> MRSMRALSLSLSIFAGAAVATTESTGKASIHDLALQKWTVTNEYGNITVPGKFPSQAHLDLHAAGVIGESNNGLNDFDLRWIAAQNWTYTSKPISGLSKHSDIATWLVFDGLDTYATVKFCDHIVGTPDNQFRQWFYDVSSALASCKSDPVLSINFGSVPRIINAINASDEVQHWPASVVYPFEYPNRQWVRKEQNDFGWDWGPAFSPVGPWQPGRIVQLSKGGELYSLNTDIDIFRKGQFNNFAPDQTAPWVVNASLDFLGTLPKHASMSVIITDASDSRSVLYSGKLEGVTQSDMTVTGSVTIDAHKPKLWWPRDMGNQQLYNITVSVSSAGSKTPILVSQRRVGFRTILFSSGNITDAQIASGITPGNNWHFEINGHEFYAKGANLIPPDAFWPRVTSDRMNRLFDSVESQNFNMLRVWSSGTYLPDWIYDIADERGVLLWSEFQFSDTLYPDSDDFKANVVGEITYNVRRLNHHASLACWMGGNEFENLMLPIAQGADPATYPYVLGQYENLFITTLFNVLAANSHSISYSPCSANNGWLEIDLDLPVPIVERYYNTTSGHIYGDTDFYNYDTSVSFDTSAYPVGRFANEFGFISMPSIQTWQQAVDPEELSFNSTTVILRNHHYPAGGLTRNIHNSTLGQVEMTLAVERYYPTPDKTDPVANFSSWCHATQLFQADMYKSEIQFYRRGSGLP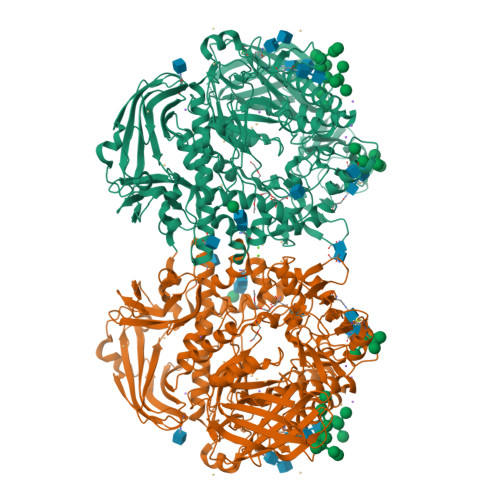ERQLGSLYWQLNDIWQAPTWAGLEYDGRWKVLPYVSRRTYEHVIASAFWNYTANELEIWVTSDLWEPVAGEVSLTWVDLKGKPIANNAGMTKSTKFNVGAINTTQIITANIQSDLKIPDTSDAVLVIELTAHGKLPNAASSKTTTFTHHNHFLPVWPNQAKVSDPKLHLSYNKSTKKFTVEATAGVSLYTWLTHPAGVLGFFDDNAFVLRPGEKKEVGFTLQQDTTGGKWTEQVTVESLWDLTTP Here we report a functional and structural genomics effort that applied saturation-level transposon mutagenesis and next generation sequencing (Tn-seq) to identify essential genes in B. thailandensis, followed by high-throughput structure determination. We used an “ortholog rescue” approach to maximize structural coverage of these gene families, which are likely to be essential not only in B. thailandensis, but also in related, but more virulent, Burkholderia species, such as B. pseudomallei. Using only seven Burkholderia species to select orthologs of essential genes, we solved structures for 49/406 essential gene families, and for 56 total Burkholderia protein targets (including seven ortholog replicates). Of these 56 targets, 25 satisfied criteria for being a potential antimicrobial drug target.

One strategy that has been employed to improve success rates is to “rescue” such proteins by adding orthologs from related species to the pipeline, based on the assumptions that many of these will have slightly different physical properties that may improve their solubility or crystallization, and that close orthologs will have structures sufficiently similar to the original target to be useful as surrogates in drug design. By using an ortholog rescue strategy for insoluble or difficult to crystallize targets, we increased our structural coverage of B. thailandensis essential genes from 31/406 (7.6%) to 49/406 (12.1%).

> MAHHHHHHMKFAFVFPGQGSQSVGMLNAFADVAVVRETLDEASDALGQDIGKLIADGPADELNLTTNTQPVMLTAAYACYRAWQQAGGAQPSIVAGHSLGEYTALVAAGAIAFRDALPLVRFRAQAMQTAVPVGVGGMAAILGLDDDTVRAVCAEASATGVVEAVNFNAPAQVVIAGTKAGIEKACEIAKEKGAKRALPLPVSAPFHSSLLKPASDKLREYLAGVDVKAPKISVVNNIDVAVVSDPAAIKDALVRQAAGPVRWVECVQHIAREGVTHVIECGPGKVLAGLTKRIDGNLVGASVFDPASLDEALKLAAA> GGCUUAUCAAGAGAGGGCGAGCGACUGGCGCGAAGAUCCCCGGCAACCAGAAAUGGUGCCAAUUCCUGCAGCGGAAACGU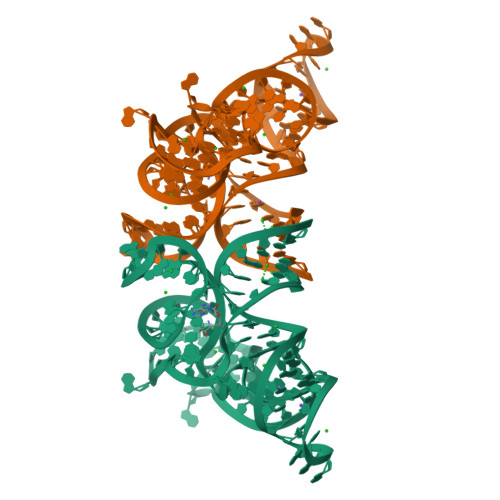UGAAAGAUGAGCCG>[2x]MSQHNILEALNVRVVGTGDRILFLAHGFGTDQSAWHLILPYFTQNYRVVLYDLVCAGSVNPDYFDFNRYTTLDPYVDDLLNIVDSLGIQNCAYVGHSVSAMIGIIASIRRPELFSKLILIGFSPRFLNDEDY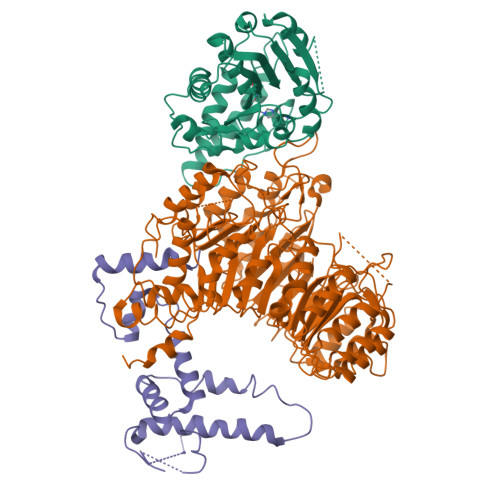HGGFEEGEIEKVFSAMEANYEAWVHGFAPLAVGADVPAAVREFSRTLFNMRPDISLFVSRTVFNSDLRGVLGLVRVPTCVIQTAKDVSVPASVAEYLRSHLGGDTTVETLKTEGHLPQLSAPAQLAQFLRRALPR;>GAMGSGIQRPTSTSSLVAAAMAEEEEVEEGRSSSSAILDLPEPLLLHILSFLTDVRSRHRAALACGRMRAAERATRSELSLRGDPRSPGFLFLSHAFRFPALEHLDLSLVSPWGHPLLSSVPPCGGGGGGAPSASSSSGMNVYHPEAISEQNAFIAARLAGCFPAVTSLAVYCRDPTTLANLTPHWQASLRRVKLVRWHQRPPTLPDGADLEPLLETCAALRELDLSEFYCWTEDVVRALTTHPSATAALTHLDLGLAAATDGFKSSELGPIAASCPNLRKLVAPCLFNPRFSDCVGDDALLSLATSCPRLTVLRLSEPFEAAANIQREEAAITVAGLVAFFAALPALEDFTMDLQHNVLEAAPAMEALARRCPRIKFLTLGSFQGLCKASWLHLDGVAVCGGLESLYMKNCQDLTDASLAAIGRGCRRLAKFGIHGCDLVTSAGIRRLAFTLRPTLKEVTVLHCRLLHTAECLTALSPIRDRIESLEINCVWNTTEQPCSVANGTTTECDPEDDELGEVYESAAKKCRYMEFDDLGSWEMLRSLSLWFSAGQLLSPLISAGLDSCPVLEEISIKVEGDCRTCPRPAPRTIFGLSDLAGFPVLAKMKLDLSEAVGYALTAPTGQMDLSLWERFYLHGIESLQTLYELDYWPPQDKDVHHRSLTLPAVGLIQRCVGLRKLFIHGTTHEHFMTFFLSIPNLRDMQLREDYYPAPENDLMFTEMRAESWLRFEVQLNSRQIDD[2x];>[2x]MDYKDDDDKMSAKKIVLKSSDGESFEVEEAVALESQTIAHMVEDDCVDNGVPLPNVTSKILAKVIEYCKRHVEAAASKAEAVEGAATSDDDLKAWDADFMKIDQATLFELILAANYLNIKNLLDLTCQTVADMIKGKTPEEIRTTFNIKNDFTPEEEEEVRRENQWAFE>MRINHNIAALNTLNRLSSNNSASQKNMEKLSSGLRINRVGDDAAGLAISEKMRGQIRGLEMASKNSQDGISLIQTAEGALTETHAILQRVRELVVQAGNTGTQDKATDLQSIQDEISALTDEIDGISNRTEFHGKKLLDGTYKVDTATPANQKNLVFQIGANATQQISVNIEDMGADALGIKEADGSIAALHSVNDLDVTKFADNAADCADIGFDAQLKVVDEAINQVSSQRAKLGAVQNRLEHTINNLSASGENLTAAESRIRDVDMAKEMSEFTKNNILSQASQAMLAQANQQPQNVLQLLR[46x]

There are three parts to the flagellar structure: the trans-membrane basal body that functions as the motor, the connecting rod and hook, and the flagellar filament that acts like a helical propeller. Our current understanding of supercoiling in bacterial flagellar filaments, referred to as polymorphic switching, is based upon the notion that protofilaments within the flagellar filament can exist in two discrete states, that differ slightly in length. The “short” state results from a protofilament having a right-handed inclination (the R-state), while the “long” state results from a protofilament having a left-handed inclination (the L-state). To reconstruct filaments at high resolution, all protofilaments must be “locked” into the same state, either L- or R-type, producing straightened filaments that lead to non-motile bacteria.

While the three L-type mutants (E115G, S285P, and S17P) have a left-handed 11-start helix, the four R-type mutants (N226Y, A233V, H84R and A39VN133H) have a right-handed 11-start helix, and the designations L and R correspond to the hand of these 11-start helices. The L-type 11-start helices are tilted left by ~ 1.7° and the R-type 11-start helices are tilted right by ~ 3.9°. Strikingly, we found those sites are not necessarily conserved among different species or participate in unique inter-subunit interactions. These include three straight mutations outside of the D1 helices: S17P, S285P (both within D0) and the double mutant A39V/N133H (within the loop region). We also identified several straight mutations that are only involved in the 11-start interactions: S17P, H84R and A39V in the double mutants. We calculated both FSC plots in the A39VN133H dataset and found that the model:map FSC (4.3 Å) is similar but more conservative compared with the map:map FSC (4.1 Å).>ALTYRGVDWSSVVVEERAGVSYKNTNGNAQPLENILAANGVNTVRQRVWVNPADGNYNLDYNIAIAKRAKAAGLGVYIDFHYSDTWADPAHQTMPAGWPSDIDNLSWKLYNYTLDAANKLQNAGIQPTIVSIGNEIRAGLLWPTGRTENWANIARLLHSAAWGIKDSSLSPKPKIMIHLDNGWDWGTQNWWYTNVLKQGTLELSDFDMMGVSFYPFYSSSATLSALKSSLDNMAKTWNKEIA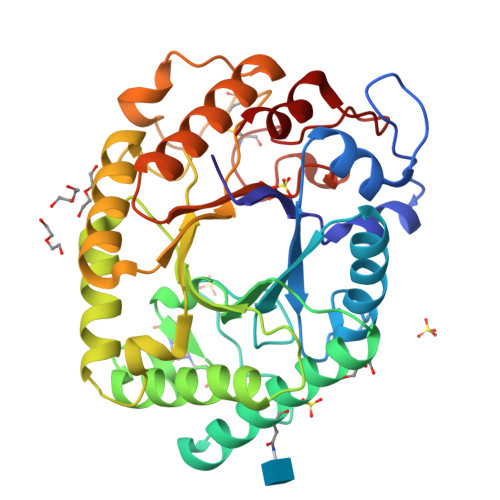VVETNWPISCPNPRYSFPSDVKNIPFSPEGQTTFITNVANIVSSVSRGVGLFYWEPAWIHNANLGSSCADNTMFSQSGQALSSLSVFQRI[4x]> DVYHDGACPEVKPVDN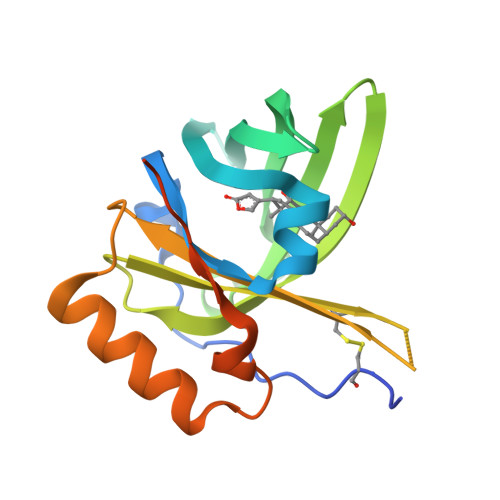FDWSQYHGKWWQVAAYPDHITKYGKCGWAEYTPEGKSVKVSRYSVIHGKEYFSEGTAYPVGDSKIGKIYHSYTIGGVTQEGVFNVLSTDNKNYIIGYFCSYDEDKKGHMDLVWVLSRSMVLTGEAKTAVENYLIGSPVVDSQKLVYSDFSEAACKVNNSNWSHPQFEK N-[3-(3-phenylisoxazol-5-yl)propanoyl]-L-alpha-glutamyl-L-alpha-glutamyl-amide 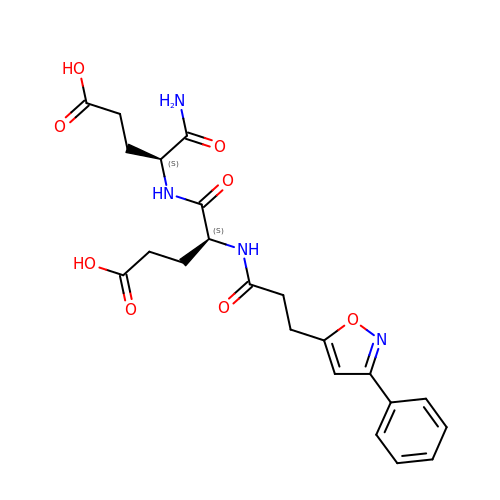| C22 H26 N4 O8 | LIIRZRQVACDFBI-HOTGVXAUSA-N> MTRLTVALSGDCMVTRGGLITSDPAAERLRDLLRGTDFAVTNLEVVPSDGRGHPVHNAVGGGCLIADSAVLDEVTAAGFSVLGCANNHAMDLGTEGVLGTMDLLRARGIPYAGIGADLTGARRPVYADRPGGSLALLSCTATFLPGQEAADPSPELPGRPGLNPLRHTATMQVTADQMDVLRTIDAETGLRARRAEARALLGVDPALLGPDRLALFGTRFRTADAPGFTTECDPRDLDEIARWVGEARLRADLVVVSVHSHEPGPTPETPGEFLRVFAHRMIDEGAHAVVGHGPHFLRGVELYRNKPIFYSLGNIVSQIELTDRVSAEDYAKVTAERPLTPGRYYDRLSGHGTRLFAPHRRYWQSLVPVLTFEDGTLTAARLHPVDLGFGRPVHRRGRPRLADRAEAEKTLTDVAQLSQPYGTAIEVMDDGTGELALDVA;> MSAVYEPPMLQEVGDFDELTKCLGVGSCNDFAGCGYAIVCFG

The lasso peptide MS-271 is a ribosomally synthesized and post-translationally modified peptide (RiPP) consisting of 21 amino acids with D-tryptophan at the C-terminus, and is derived from the precursor peptide MslA. MslH, encoded in the MS-271 biosynthetic gene cluster (msl), catalyzes the epimerization at the Cα center of the MslA C-terminal Trp21, leading to epi-MslA. Herein, based on X-ray crystallographic studies in association with MslA core peptide analogues, we show that MslH is a metallo-dependent peptide epimerase with a calcineurin-like fold. The crystal structure analysis, followed by site-directed mutagenesis, docking simulation, and ICP-MS studies demonstrate that MslH employs acid/base chemistry to facilitate the reversible epimerization of the C-terminal Trp21 of MslA, by utilizing two pairs of His/Asp catalytic residues that are electrostatically tethered to a six-coordination motif with a Ca(II) ion via water molecules.

Hence, recombinant N-terminally His6-tagged MslAΔTrp21, which lacked the C-terminal Trp21, and MslA Trp21G variants, with an achiral glycine instead of Trp21, were prepared by co-expression with MslB1 in E. coli. As a result, the X-ray crystal structures of the MslH:MslAΔTrp21 and MslH:MslA Trp21G complexes at 2.29 Å and 2.12 Å resolutions, respectively, with one monomer in the asymmetric unit, which are the same as the MslH:apo structure, were successfully obtained. In a manner similar to the MslH:MslAΔTrp21 structure, the MslH:MslA Trp21G structure accommodated the MslA Trp21G molecule, consisting of the Gly12-Tyr15 and Cys19-Gly21 parts on the C-terminal side of MslA Trp21G with a disulfide bond between Cys13 and Cys19, in the large cleft. In addition, the amide nitrogen and oxygen atoms between Phe20 and Gly21 in MslA Trp21G formed polar interactions with the oxygen atom in the backbone of MslH Gly60 and the nitrogen atom of the His295 side chain, respectively (2.6 Å and 2.5 Å). Because the amide bond was recognized by MslH in a similar manner to the carboxyl group of the C-terminal MslA Phe20, the electron densities of MslA analogues likely represented the binding mode of the original MslA substrate in MslH. The structure analyses also revealed that the C-terminal MslA Phe20 carboxyl group in MslAΔTrp21 and the C-terminal MslA Phe20 and Gly21 in MslA Trp21G are located near a hydrophobic pocket consisting of MslH Gly60-62 and Leu64 on the core domain and Ile319, Tyr345, Leu348, Leu355, and Phe356 on the C-domain in monomer A at the edge of the cleft, respectively. In addition, an architecture that would construct a six-coordination motif, consisting of four amino acid residues Glu44, Asn87, His259, and His261 and two water molecules (w1 and w2), was detected around the C-terminal carboxyl group of MslA Phe20 in the MslH:MslAΔTrp21 crystal structure.> SHMELTPDQQTLLHFIMDSYNKQRMPQEITNKILKEEFSAEENFLILTEMATNHVQVLVEFTKKLPGFQTLDHEDQIALLKGSAVEAMFLRSAEIFNKKLPSGHSDLLEERIRNSGISDEYITPMFSFYKSIGELKMT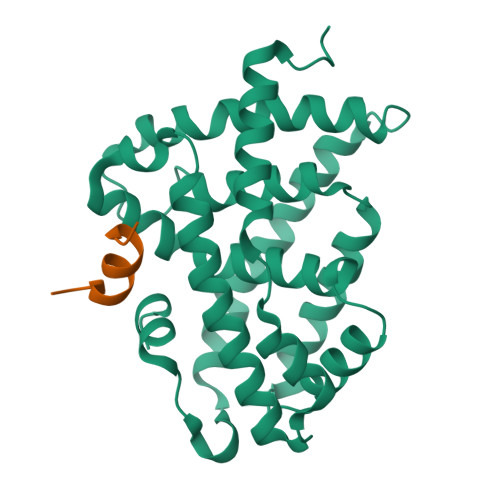QEEYALLTAIVILSPDRQYIKDREAVEKLQEPLLDVLQKLCKIHQPENPQHFACLLGRLTELRTFNHHHAEMLMSWRVNDHKFTPLLCEIWDVQ;> KENALLRYLLDKD>[2x]MDRNS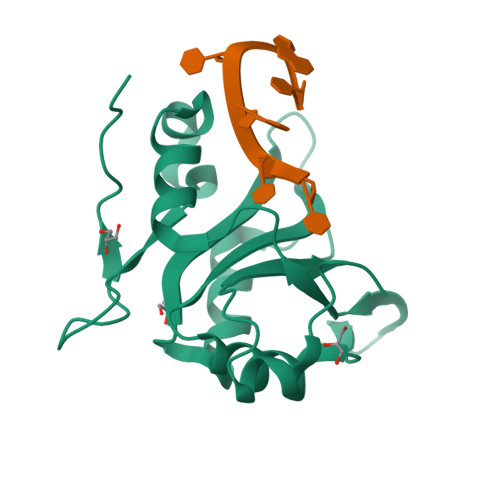VDYAQIASGIDTRTTVMIKNIPNKFTQQMLRDYIDVTNKGTYDFLYLRIDFVNKCNVGYAFINFIEPQSIITFGKARVGTQWNVFHSEKICDISYANIQGKDRLIEKFRNSCVMDENPAYRPKIFVSHGPNRGMEEPFPAPNNARRKLRS> GSMPVRRGHVAPQNTFLDTIIRKFEGQSRKFIIANARVENCAVIYCNDGFCELCGYSRAEVMQRPCTCDFLHGPRTQRRAAAQIAQAL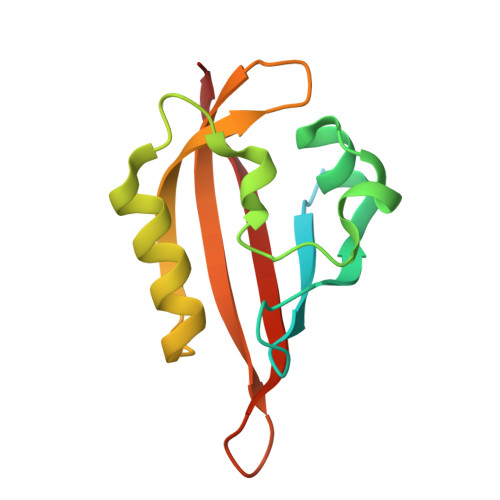LGAEERKVEIAFYRKDGSCFLCLVDVVPVKNEDGAVIMFILNFEVVMEK> MPELEVKGKKL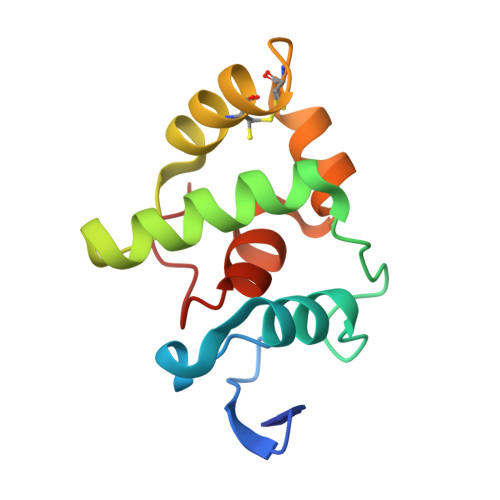RLDEDGFLQDWEEWDEEVAEALAKDTRFSPQPIELTEEHWKIIRYLRDYFIKYGVAPPVRMLVKHCKKEVRPDCNLQYIYKLFPQGPAKDACRIAGLPKPTGCV2-[[3-(3-methoxyphenyl)phenyl]-(4-pyridyl)methyl]guanidine 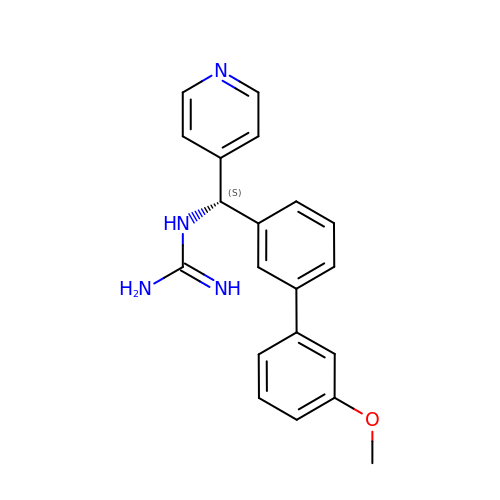| C20 H20 N4 O | LSPQISZRKHVJOD-LJQANCHMSA-N> MAKTLKDLQGWEIITTDEQGNIIDGGQKRLRRRGNKTEHYLKRSSDGIKLGRGDSVVMHNEAAGTYSVYMIQELRLNTLNNVVELWALTYLRWFEVNPLAHYRQFNPDANILNRPLNYYNKLFSETANKNELYLTAELAELQLFNFIRVANVMDGSKWEVLKGNVDPE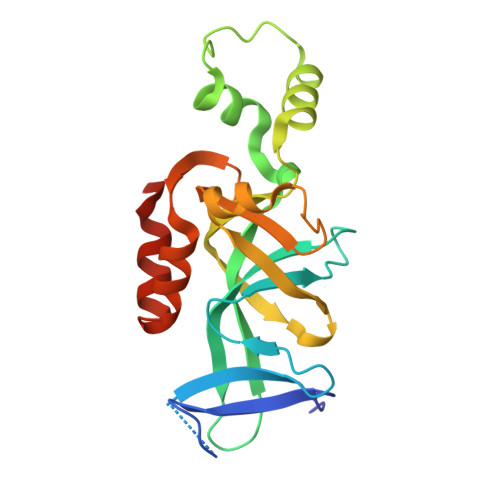RDFTVRYICEPTGEKFVDINIEDVKAYIKKVEPREAQEYLKDLTLPSKKKE>MAHHHHH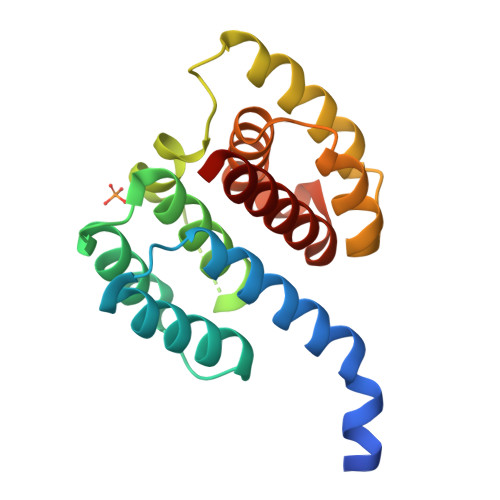HSSGLEVLFQGPMSLLTEVETYVLSIVPSAPLKAEIAQRLEDVFAGKNTDLEVLMEWLKTRPILSPLTKGILGFVFTLTVPSERGLQRRRFVQNALNGNGDPNNMDKAVKLYRKLKREITFHGAKEIALSYSAGALASCMGLIYNRMGAVTTEVAFGLVCATCEQIADSQ[2x]>MSNVFYRSSKPYPVAVRGEGVFLYDDAGRRYLDGSSGALVANIGHGRAEVGERMAAQAARLPFVHGSQFSSDVLEEYAGRLARFVGLPTFRFWAVSGGSEATESAVKLARQYHVERGEPGRFKVITRVPSYHGASLGSLAASGMGARRELYTPLMRPEAWPKLPKPDPARNGAEDAEGLRALLEREGPETVAAFMAEPVVGASDAALAPAPGYYERVRDICDEAGIIFIADEVMSGMGRCGSPLALSRWSGVTPDIAVLGKGLAAGYAPLAGLLAAPQVYETVMGGSGAFMHGFTYAGHPVSVAAGLSVLDIVEREDLTGAAKERGAQLLAGLQALQARFPQMMQVRGTGLLLGVVLGDLATGQAFETPGIASRIGAAALKRGLITYPGSGA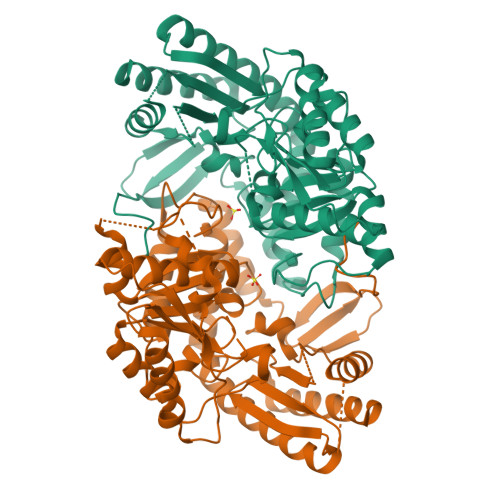EPNGRGDHLLLGPPLSITAAEVDGLLALLAGALEDVLG[4x]4-[2-(HYDROXYMETHYL)PYRIMIDIN-4-YL]-N,N-DIMETHYLPIPERAZINE-1-SULFONAMIDE 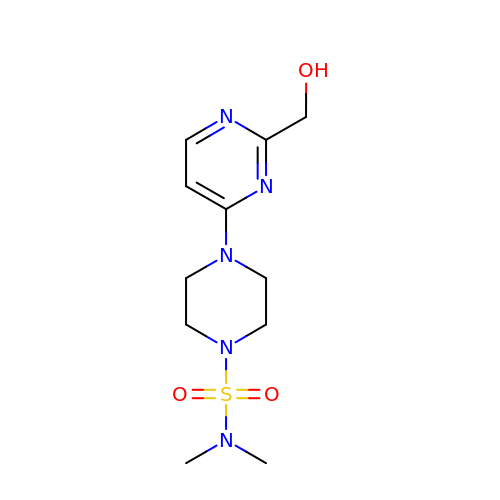| C11 H19 N5 O3 S | XDTHNROWHAAVPJ-UHFFFAOYSA-N>[2x]MIELSLAEALFLILFTGVISMLISRRTGISYVPIFILTGLVIGPLLKLIPRDLAHEIFDFVRVFGLVIILFTEGHNLSWRLLKKNMPTIVTLDTIGLILTALIAGFIFKVVFNSSFLLGFLFGAIIGATDPATLIPLFRQYRVKQDIETVIVTESIFNDPLGIVLTLIAISMLVPGYGGGIFSTLSEKLGIYAGGVIYFLYNVSVSISLGIFLGILGYKFIKRTGIFDFPEI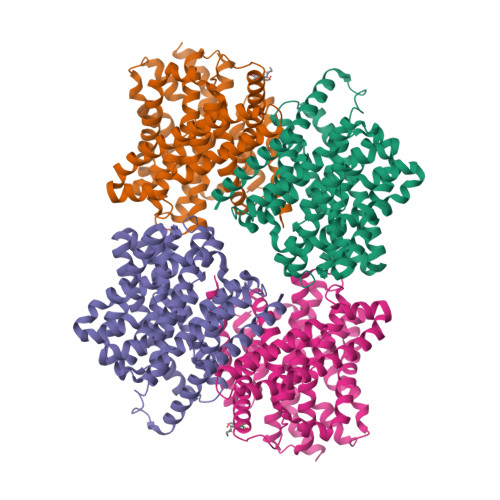EAFSLSLAFLGFFIGERLDASGYLVATVTGIVLGNYKLLKPRENIRILKRLQRAIEKEVHFNDTLAALATIFIFVLLGAEMNLEVIWSNLGKGLLVALGVMILARPLATLPLLKWWNFREYLFIALEGPRGVVPSALASLPLSLALKYKSPLLTVHWGEIIMATVVITVLTSVIVETLWIPILKDKLDVG6-ETHYL-CHENODEOXYCHOLIC ACID | C26 H44 O4 | 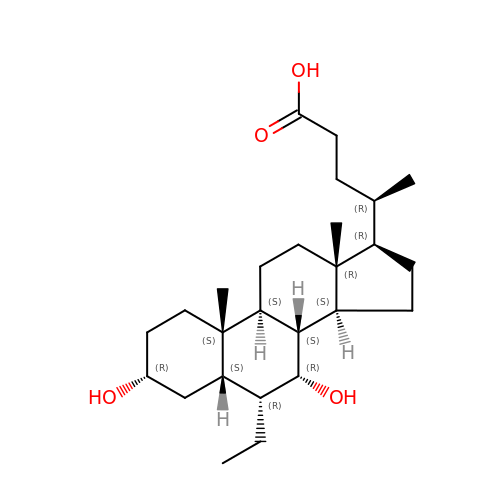ZXERDUOLZKYMJM-ZWECCWDJSA-N> HEDEIKKLRTSGSMTQNPHEVARVRNLNRIIMGKYEIEPWYFSPYPIELTDEDFIYIDDFTLQYFGSKKQYERYRKKCTLRHPPGNEIYRDDYVSFFEIDGRKQRTWCRNLCLLSKLFLDHKTLYYDVDPFLFYCMTRRDELGHHLVGYFSKEKESADGYNVACILTLPQYQRMGYGKLLIEFSYELSKKENKVGSPQKPLSDLGLLSYRAYWSDTLITLLVEHQKEITIDEISSMTSMTTTDILHTAKTLNILRYYKGQHIIFLNEDILDRYNRLKAKKRRTIDPNRLIWKPPVFTASQLRFA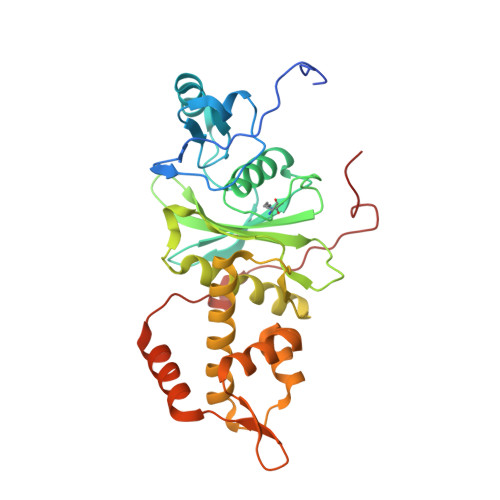W>MTNRQWETLREYDEIKYEFYEGIAKVTINRPEVRNAFTPKTVAEMIDAFSRARDDQNVSVIVLTGEGDLAFCSGGDQKKRGHGGYVGEDQIPRLNVLDLQRLIRIIPKPVIAMVKGYAVGGGNVLNVVCDLTIAADNAIFGQTGPKVGSFDAGYGSGYLARIVGHKKAREIWYLCRQYNAQEALDMGLVNTVVPLEKVEDETVQWCKEIMKHSPTALRFLKAAMNADTDGLAGLQQMAGDATL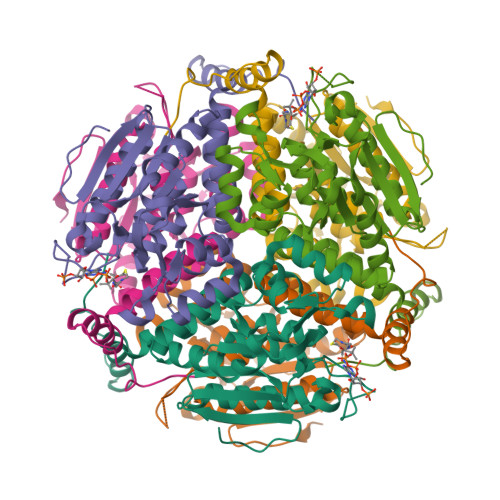LYYTTDEAKEGRDAFKEKRDPDFDQFPKFP[2x]> GASSDKIIHLTDDSFDTDVLKADGAILVDFWAEWCGPCKMIAPILDEIADEYQGKLTVAKLNIDQNPGTAPKYGIRGIPTLLLFKNGEVAAT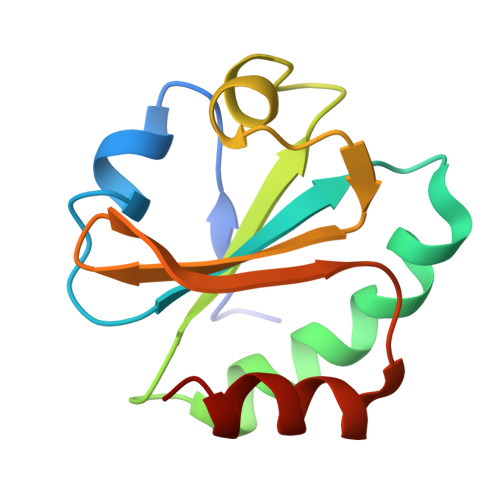KVGALSKGQLKEFLDANLA> DLSLSDINSTVEVPEGHSFWKTLLAYSGPGALVAVGYMDPGNWSTSITGGQNFQYLLLSIIVISSLLAMLLQNMAAKLGIVCQLDLAQAIRARTSRRLGFIFWILTELAIMATDIAEVIGAAIALYLLFKIPIFLAVVITVLDVFLLLLLNRIGFRKIEALVVCLIFVILFVFLYQIILSQPAWHQVAKGLIPSWASVQTSPKIGGQTPLSASLGIIGATIMPHNLFLHSAISQSRKIDRTDSSKVAEAVRFSNWDSNIQLSLAMVVNALLLIMGVAVFKSGAVQDPSFFGLYQALSNPDMVSNPVLAEAARSGVLSTLFAVALLASGQNSTITGTITGQVIMEGFIHLRLPLWLRRLVTRLIAIIPVVVCV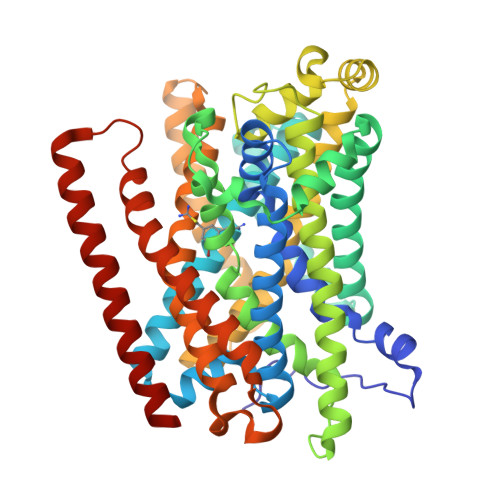AITSHQGSLDEHQALNNLMNNSQVFLALALPFSIVPLLMLTDSAAQMGNQFKNTRWVKVMGWLTVIILTLLNLISISSQIAGFFGDNPSSQDLLLSQVISIGIILAMIGLLIWTIIDIRRFT>[4x]MWERDRVIVLGHRGYMSNYPENTLLAFRKAVEAGADGIELDVWLTKDGRVVVMHDETIDRTSNMKGRQKDMTLEELKKADVGQGERIPTLEEVFEAI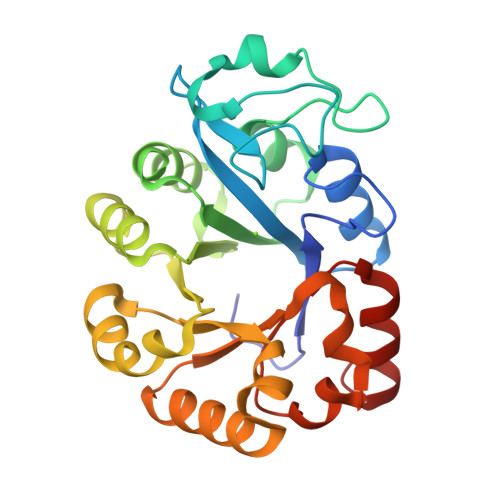PRNALVNVELKDRDAAREVAEIVAENNPERVMISSFDIDALREYRKYDDETTMGLLIDREEVVPLIPKLKDELNLWSVNVPMEAIPLIGLEKTLQALHWVRSLGLKVVLWTENDVLFYKDDNLAKLKGLFEVVIANDVVRMIEYLKKLGLR> MGHHHHHHMLHLLEQIRAYCETCWEWQEAHEPGMDQDKNPMPAPVEHQICPAVCVLM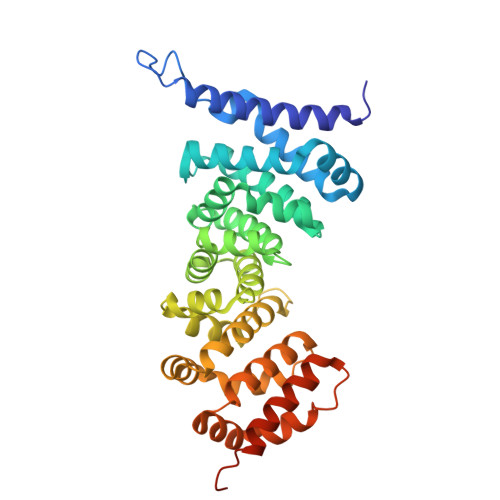KLSFDEEHRHAMNELGGLQAIAELLQVDCEMYGLTNDHYSITLRRYAGMALTNLTFGDVANKATLCSMKGCMRALVAQLKSESEDLQQVIASVLRNLSWRADVNSKKTLREVGSVKALMECALEVKKESTLKSVLSALWNLSAHCTENKADICAVDGALAFLVGTLTYRSQTNTLAIIESGGGILRNVSSLIATNEDHRQILRENNCLQTLLQHLKSHSLTIVSNACGTLWNLSARNPKDQEALWDMGAVSMLKNLIHSKHKMIAMGSAAALRNLMANRPAKYKDANIMSPGSSLPS> KMSMSTMNMPMAMKVGGGGSGGGGSGGGGSSAFFFCGAIFECHYLNGTERVRYLQRYIYNRQQLVHFDSDVGKFVADTPLGEPQAEYWNSNAELLENIMNIADGSCRHNYGILESFTVQRSVEPKVRVSALQSGSLPETDRLACYVTGFYPPEIEVKWFLNGREETERVVSTD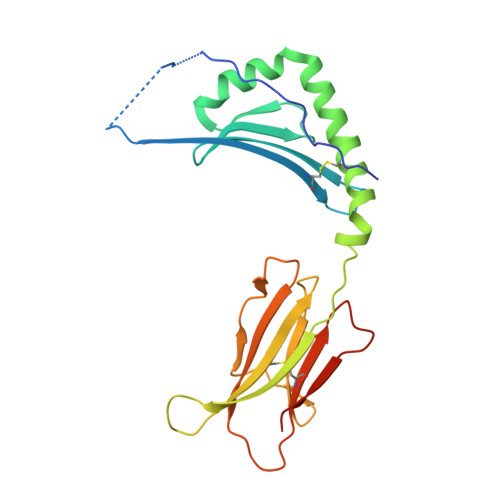VMQNGDWTYQVLVVLETVPRRGDSYVCRVEHASLRQPISQAWEPPADAGRSK N-{2-[4-(AMINOSULFONYL)PHENYL]ETHYL}ACETAMIDE | C10 H14 N2 O3 S | 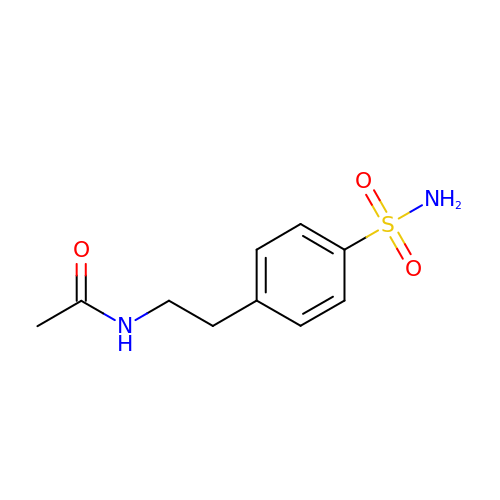IIMGUEXQORZTID-UHFFFAOYSA-N> MRINHNIAALNTLNRLSSNNSASQKNMEKLSSGLRINRAGDDAAGLAISEKMRGQIRGLEMASK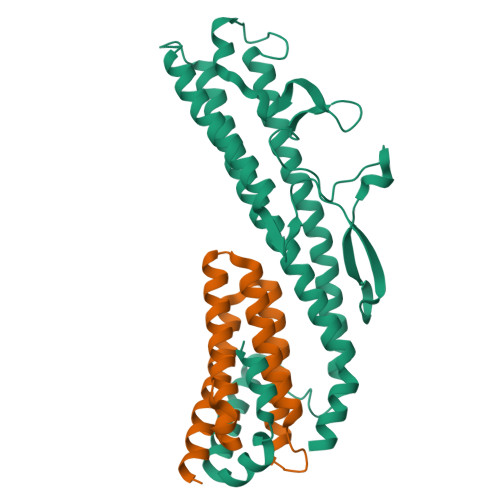NSQDGISLIQTAEGALTETHAILQRVRELVVQAGNTGTQDKATDLQSIQDEISALTDEIDGISNRTEFNGKKLLDGTYKVDTATPANQKNLVFQIGANATQQISVNIEDMGADALGIKEADGSIAALHSVNDLDVTKFADNAADTADIGFDAQLKVVDEAINQVSSQRAKLGAVQNRLEHTINNLSASGENLTAAESRIRDVDMAKEMSEFTKNNILSQASQAMLAQANQQPQNVLQLLR;> MAIQNPYTAYQQNSVNTATPGELTLMLYNGCLKFIRLAAQAIENDDMERKNENLIKAQNIIQELNFTLNRNIELSASMGAMYDYMYRRLVQANIKNDTGMLAEVEGYVTDFRDAWKQAIQSERKDRHGSGGIA>[2x]SATLKVSDSVPAPSDDAEQLRTAFEGWGTNEDLIISILAHRSAEQRKVIRQAYHETYGEDLLKTLDKELSNDFERAILLWTLEPGERDALLANEAT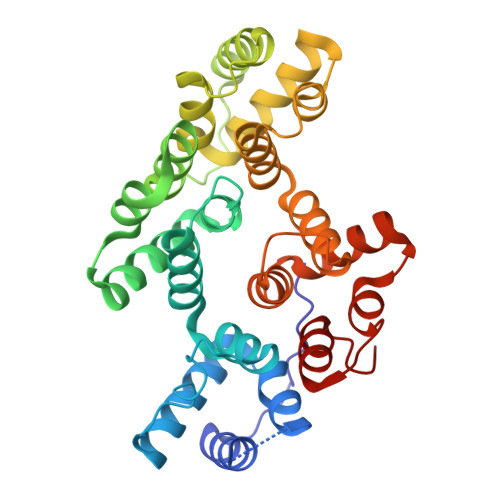KRWTSSNQVLMEVACTRTSTQLLHARQAYHARYKKSLEEDVAHHTTGDFRKLLVSLVTSYRYEGDEVNMTLAKQEAKLVHEKIKDKHYNDEDVIRILSTRSKAQINATFNRYQDDHGEEILKSLEEGDDDDKFLALLRSTIQCLTRPELYFVDVLRSAINKTGTDEGALTRIVTTRAEIDLKVIGEEYQRRNSIPLEKAITKDTRGDYEKMLVALLGEDDA2-[4-oxidanylidene-3-(2-phenylethyl)pteridin-2-yl]sulfanyl-~{N}-(1,3-thiazol-2-yl)ethanamide 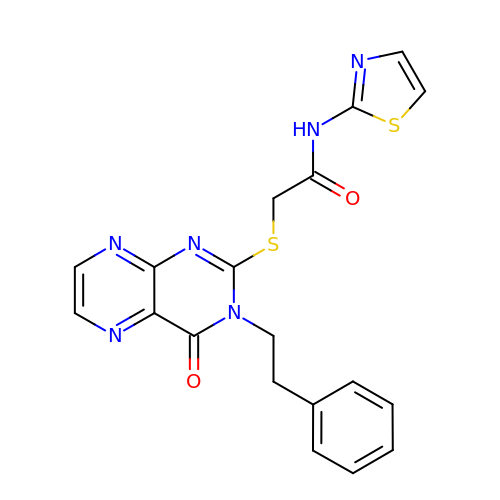| C19 H16 N6 O2 S2 | ANHMCIKPOJARRV-UHFFFAOYSA-N> MDRLDRKILRILQEDSTLAVADLAKKVGLS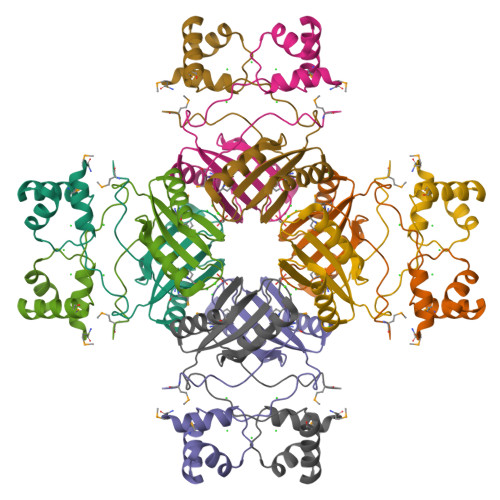TTPCWRRIQKMEEDGVIRRRVALLDPVKVNTKVTVFVSIRTASHSIEWLKRFSEVVSEFPEVVEFYRMSGDVDYLLRVVVPDIAAYDAFYKRMIAKIEIRDVSSAFAMEQIKYTTELPLDYMLLDNPKSGEE> FEKCGKRVDRLDQRRSKL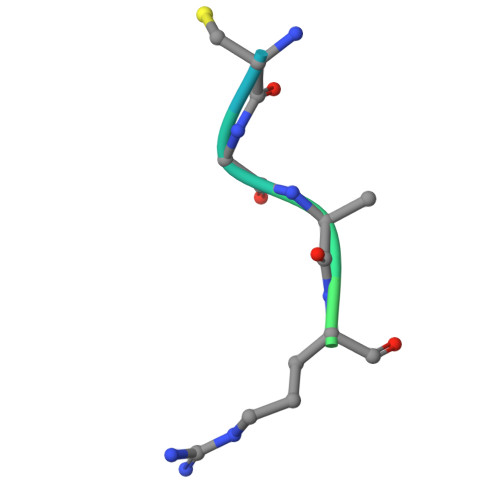R>MNLTELKNTPVSELITLGENMGLENLARMRKQDIIFAILKQHAKSGEDIFGDGVLEILQDGFGFLRSADSSYLAGPDDIYVSPCQIRRFNLRTGDTISGKIRPPKEGERYFALLKVNEVNFDKPENARNKILFENLTPLHANSRLRMERGNGSTEDLTARVLDLASPIGRGQRGLIVAPPKAGKTMLLQNIAQSIAYNHPDCVLMVLLIDERPEEVTEMQRLVKGEVVASTFDEPASRHVQVAEMVIEKAKRLVEHKKDVIILLDSITRLARAYNTVVPASGKVLTGGVDANALHRPKRFFGAARNVEEGGSLTIIATALIDTGSKMDEVIYEEFKGTGNMELHLSRKIAEKRVFPAIDYNRSGTRKEELLTTQEELQKMWILRKIIHPMGEIDAMEFLINKLACTKTNDDFFEMMKR[12x]

Bacterial RNA helicase ρ is a genome sentinel that terminates the synthesis of damaged and junk RNAs that are not translated by the ribosome. The N-terminal domain (NTD) contains a primary RNA-binding site (PBS), the C-terminal domain (CTD) harbors a secondary RNA-binding site (SBS) and ATPase and helicase modules. Our results demonstrate that ADP and (p)ppGpp nucleotides bound at subunit interfaces inhibit ρ ring closure that underpins the hexamer activation, thus favoring the assembly of inactive higher-order oligomers. Here, we show that stress-associated nucleotides ADP and (p)ppGpp bind to the nucleotide-binding site in the CTD to trigger the formation of inactive ρ aggregates.

To test whether ρ forms filaments as revealed by the structures, we designed “sensor” Cys residues that would be closely spaced in filaments and used bismaleimidoethane (BMOE), a high-efficiency short-length (8.0 Å) cell-permeable sulfhydryl-to-sulfhydryl crosslinker, to assess filament formation. By contrast, (p)ppGpp induces the formation of transient ρ dodecamers. Our crosslinking shows that ADP, but not (p)ppGpp, promotes the formation of extended ρ filaments and our structures suggest that ADP-filaments may be more stable than ppGpp-induced dodecamers. Indeed, we observed that ppGpp-induced crosslinking of S84C ρ is incompatible with the filament structure. To corroborate this idea, we obtained a structure of ρX1 that was BMOE-crosslinked in the presence of ppGpp. Our results demonstrate that, in the presence of (p)ppGpp, the majority of ρ forms transient “non-extendable” dodecamers that cannot give rise to filaments and co-exist with a minor fraction of the filament-competent state. The alternative C-to-N filament and N-to-N constellations might explain the two bands representing dodecamers observed after BMOE crosslinking. Residue substitutions in the linker that connects ρ domains or binding of stress-associated nucleotides to the nearby ATPase site trigger the formation of dodecamers and higher-order polymers. ρ hexamers can form dynamic N-to-N dimers and long C-to-N filaments, which can be visualized by crosslinking in the presence of (p)ppGpp and ADP, respectively. Formation of stable (for cryoEM analyses) N-to-N dimers required prior crosslinking, and long ρ filaments could be directly observed on EM grids only if additionally stabilized by the C-terminal H8 extension and linker substitutions.D-TYROSINE | C9 H11 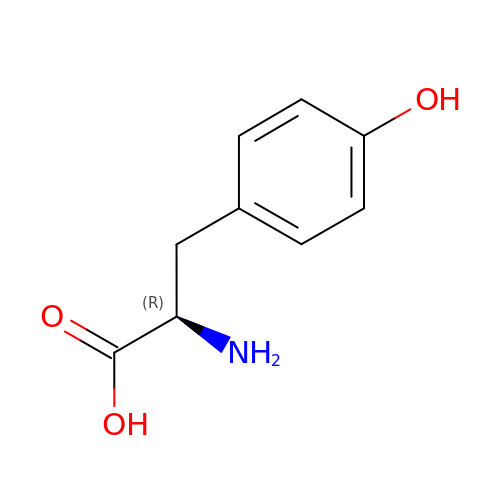N O3 | OUYCCCASQSFEME-MRVPVSSYSA-N>GYINAAFRSSRNNEAYLFINDKYVLLDYAPGTSNDKVLYGPSFVRDGYKSLAKTIFGTYGIDCSFDTEYNEAFIFYENFCARIDYAPHSDKDKIISGPKKIADMFPFFKGTVFENGIDAAFRSTKGKEVYLFKGDKYARIDYLTNRLVQNIKSISDGFPC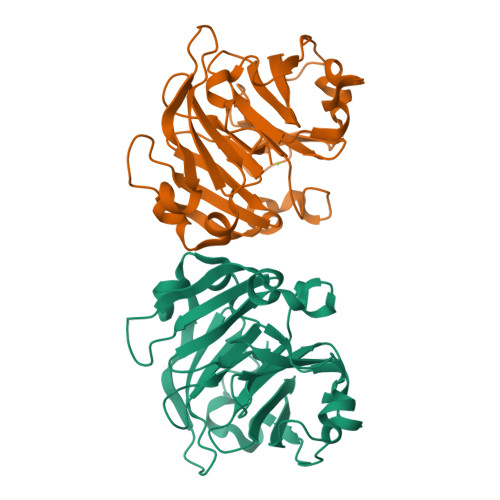LRGTIFEAGMDSAFASHKTNEAYLFKGEYYARINFTPGSTNDIMGGVKKTLDYWPSLRGIIPLE[2x]>[2x]GHMKGNTMKQLRFGLFENAQTNDSGTATWRHPDNQRHLFDTLDYWRNIAQICEDAGLDFVFLADA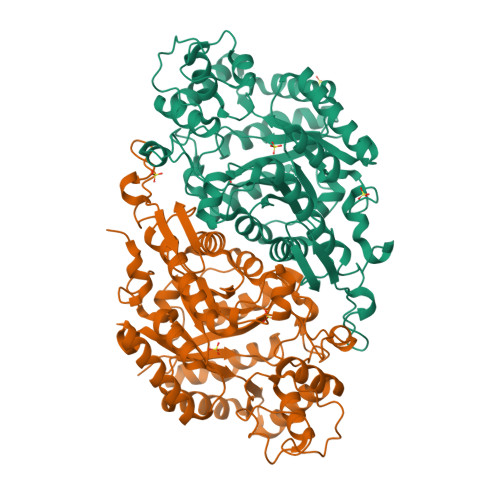WGWADVNGERPDICDVEGLDLPRLDPAIVAAALIASTTKLGLVMTGSTLLEQPYSFARRMASLDHLSKGRIGWNVVTTGTAETASAAFGVPMVAHDDRYDMADDFMELVYKLWEGAWEPDALERDKQGRYADPAKVHRIDHEGPYFRSNGYGNTSYSPQGTPVLFQAGSSERGRQFGGRHGECIFLGGAPIPKLAEQVRAIRAEAVAEGRAADSIKLMAAFSCVIAPTHEEAVQKYQEVLDSQTPEVAVASYAWFTGLDLSSYDPSTPMSELHTELSQTQVARFAGLTVGDVLADWHAHGVRTKPVVGTPEEVADAIVELAEGADLDGFLLTPVIQPGSTIDFIEHVLPILRERGVAASGYDAPTLRERLLGTETPVLREDHPGAGYRAQSGALVG> MHHHHHHAADPPPVHDTDGHELRADANYYVLSANRAHGGGLTMAPGHGRHCPLFVSQDPNGQHDGFPVRITPYGVAPSDKIIRLSTDVRISFRAYTTCLQSTEWHIDSELAAGRRHVITGPVKDPSPSGRENAFRIEKYSGAEVHEYK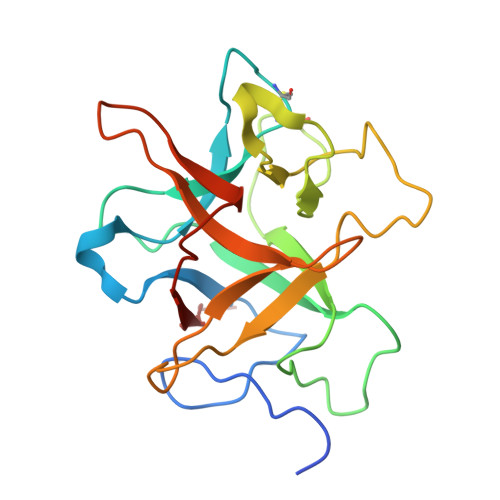LMSSGDWCQDLGVFRDLKGGAWFLGATEPYHVVVFKKAPPA> DYNGQAKCMLEKVGNWNFDIFLFDRLTNGNSLVSLTF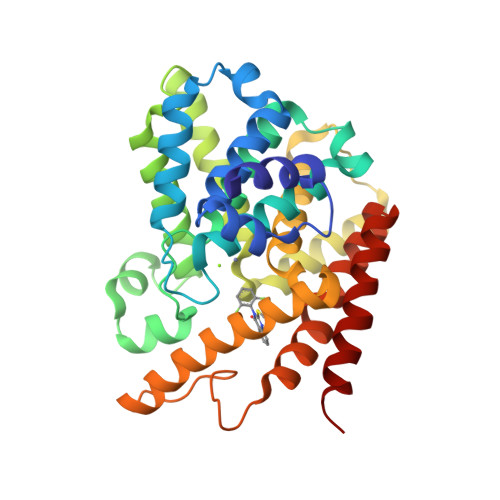HLFSLHGLIEYFHLDMMKLRRFLVMIQEDYHSQNPYHNAVHAADVTQAMHCYLKEPKLANSVTPWDILLSLIAAATHDLDHPGVNQPFLIKTNHYLATLYKNTSVLENHHWRSAVGLLRESGLFSHLPLESRQQMETQIGALILATDISRQNEYLSLFRSHLDRGDLCLEDTRHRHLVLQMALKCADICNPCRTWELSKQWSEKVTEEFFHQGDIEKKYHLGVSPLCDRHTESIANIQIGFMTYLVEPLFTEWARFSNTRLSQTMLGHVGLNKASWKGLQR>[2x]MPTQSKHASINIGLIQAREALMTQFRPILNQA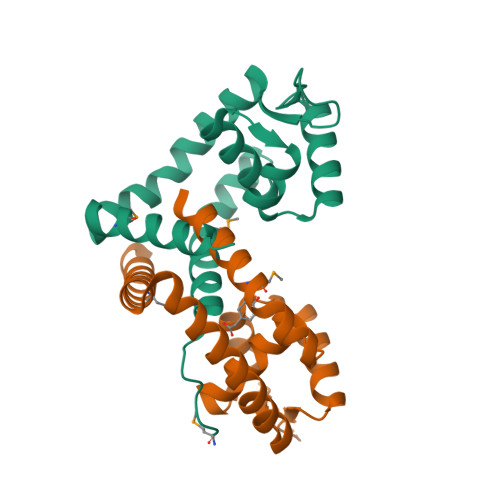NITDQQWRIIRLLAENGTLDFQDLANQACILRPSLTGILTRLEKAGLVVRLKPSNDQRRVFLKLTAEGEKLYEEIGEEVDERYDAIEEVLGREKMLLLKDLLAELAKIEDALNS> MPFVNKQFNYKDPVNGVDIAYIK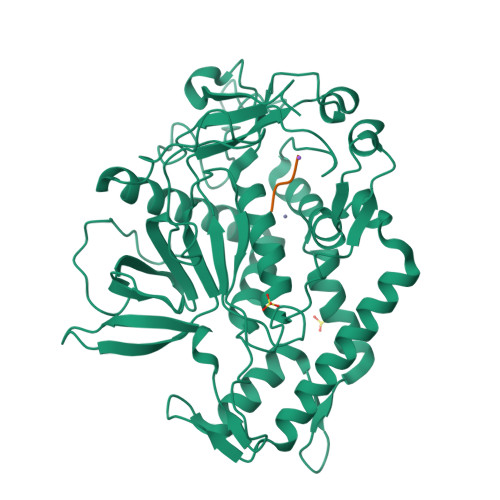IPNAGQMQPVKAFKIHNKIWVIPERDTFTNPEEGDLNPPPEAKQVPVSYYDSTYLSTDNEKDNYLKGVTKLFERIYSTDLGRMLLTSIVRGIPFWGGSTIDTELKVIDTNCINVIQPDGSYRSEELNLVIIGPSADIIQFECKSFGHEVLNLTRNGYGSTQYIRFSPDFTFGFEESLEVDTNPLLGAGKFATDPAVTLAHELIHAGHRLYGIAINPNRVFKVNTNAYYEMSGLEVSFEELRTFGGHDAKFIDSLQENEFRLYYYNKFKDIASTLNKAKSIVGTTASLQYMKNVFKEKYLLSEDTSGKFSVDKLKFDKLYKMLTEIYTEDNFVKFFKVLNRKTYLNFDKAVFKINIVPKVNYTIYDGFNLRNTNLAANFNGQNTEINNMNFTKLKNFTGLFELEHHHHHH;> RRGCX> MDYKDDDDKLAAANSSIDLISTSLYKKAGFKGTNSVDMKVDRTKLKKTPTEAPADCRALIDKLKVCNDEQLLLELQQIKTWNIGKCELYHWVDLLDRFDGILADAGQTVENMSWMLVCDRPEREQLKMLLLAVLNFTALLIEYSFSRHLYSSIEHLTTLLASSDMQVVLAVLNLLYVFSKRSNYITRLGSDKRTPLLTRLQHLAESWGGKENGFGLAECCRDLHMMKYPPSATTLHFEFYADPGAEVKIEKRTTSNTLHYIHIEQLDKISESPSEIMESLTKMYSIPKDKQMLLFTHIRLAHGFSNHRKRLQAVQARLHAISILVYSNALQESANSILYNGLIEELVDVLQITDKQLMEIKAASLRTLTSIVHLERTPKLSSIIDCTGTASYHGFLPVLVRNCIQAMIDPSMDPYPHQFATALFSFLYHLASYDAGGEALVSCGMMEALLKVIKFLGDEQDQITFVTRAVRVVDLITNLDMAAFQSHSGLSIFIYRLEHEVDLCRKECPFVIKPKIQRPNTTQEGEEMETDMDGVQCIPQRAALLKSMLNFLKKAIQDPAFSDGIRHVMDGSLPTSLKHIISNAEYYGPSLFLLATEVVTVFVFQEPSLLSSLQDNGLTDVMLHALLIKDVPATREVLGSLPNVFSALCLNARGLQSFVQCQPFERLFKVLLSPDYLPAMRRRRSSDPLGDTASNLGSAVDELMRHQPTLKTDATTAIIKLLEEICNLGRDPK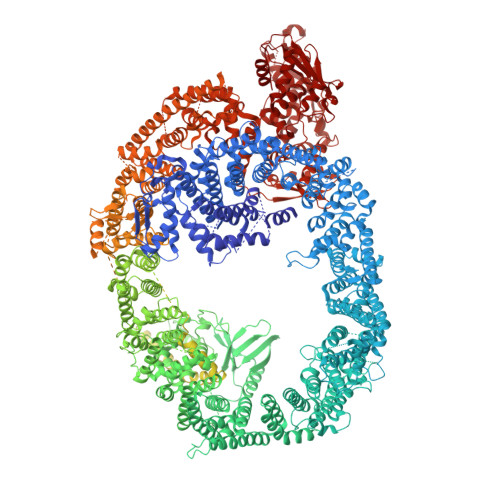YICQKPSIQKADGTATAPPPRSNHAAEEASSEDEEEEEVQAMQSFNSTQQNETEPNQQVVGTEERIPIPLMDYILNVMKFVESILSNNTTDDHCQEFVNQKGLLPLVTILGLPNLPIDFPTSAACQAVAGVCKSILTLSHEPKVLQEGLLQLDSILSSLEPLHRPIESPGGSVLLRELACAGNVADATLSAQATPLLHALTAAHAYIMMFVHTCRVGQSEIRSISVNQWGSQLGLSVLSKLSQLYCSLVWESTVLLSLCTPNSLPSGCEFGQADMQKLVPKDEKAGTTQGGKRSDGEQDGAAGSMDASTQGLLEGIGLDGDTLAPMETDEPTASDSKGKSKITPAMAARIKQIKPLLSASSRLGRALAELFGLLVKLCVGSPVRQRRSHHAASTTTAPTPAARSTASALTKLLTKGLSWQPPPYTPTPRFRLTFFICSVGFTSPMLFDERKYPYHLMLQKFLCSGGHNALFETFNWALSMGGKVPVSEGLEHSDLPDGTGEFLDAWLMLVEKMVNPTTVLESPHSLPAKLPGGVQNFPQFSALRFLVVTQKAAFTCIKNLWNRKPLKVYGGRMAESMLAILCHILRGEPVIRERLSKEKEGSRGEEDTGQEEGGSRREPQVNQQQLQQLMDMGFTREHAMEALLNTSTMEQATEYLLTHPPPIMGGVVRDLSMSEEDQMMRAIAMSLGQDIPMDQRAESPEEVACRKEEEERKAREKQEEEEAKCLEKFQDADPLEQDELHTFTDTMLPGCFHLLDELPDTVYRVCDLIMTAIKRNGADYRDMILKQVVNQVWEAADVLIKAALPLTTSDTKTVSEWISQMATLPQASNLATRILLLTLLFEELKLPCAWVVESSGILNVLIKLLEVVQPCLQAAKEQKEVQTPKWITPVLLLIDFYEKTAISSKRRAQMTKYLQSNSNNWRWFDDRSGRWCSYSASNNSTIDSAWKSGETSVRFTAGRRRYTVQFTTMVQVNEETGNRRPVMLTLLRVPRLNKNSKNSNGQELEKTLEESKEMDIKRKENKGNDTPLALESTNTEKETSLEETKIGEILIQGLTEDMVTVLIRACVSMLGVPVDPDTLHATLRLCLRLTRDHKYAMMFAELKSTRMILNLTQSSGFNGFTPLVTLLLRHIIEDPCTLRHTMEKVVRSAATSGAGSTTSGVVSGSLGSREINYILRVLGPAACRNPDIFTEVANCCIRIALPAPRGSGTASDDEFENLRIKGPNAVQLVKTTPLKPSPLPVIPDTIKEVIYDMLNALAAYHAPEEADKSDPKPGVMTQEVGQLLQDMGDDVYQQYRSLTRQSSDFDTQSGFSINSQVFAADGASTETSASGTSQGEASTPEESRDGKKDKEGDRASEEGKQKGKGSKPLMPTSTILRLLAELVRSYVGIATLIANYSYTVGQSELIKEDCSVLAFVLDHLLPHTQNAEDKDTPALARLFLASLAAAGSGTDAQVALVNEVKAALGRALAMAESTEKHARLQAVMCIISTIMESCPSTSSFYSSATAKTQHNGMNNIIRLFLKKGLVNDLARVPHSLDLSSPNMANTVNAALKPLETLSRIVNQPSSLFGSKSASSKNKSEQDAQGASQDSSSNQQDPGEPGEAEVQEEDHDVTQTEVADGDIMDGEAETDSVVIAGQPEVLSSQEMQVENELEDLIDELLERDGGSGNSTIIVSRSGEDESQEDVLMDEAPSNLSQASTLQANREDSMNILDPEDEEEHTQEEDSSGSNEDEDDSQDEEEEEEEDEEDDQEDDEGEEGDEDDDDDGSEMELDEDYPDMNASPLVRFERFDREDDLIIEFDNMFSSATDIPPSPGNIPTTHPLMVRHADHSSLTLGSGSSTTRLTQGIGRSQRTLRQLTANTGHTIHVHYPGNRQPNPPLILQRLLGPSAAADILQLSSSLPLQSRGRARLLVGNDDVHIIARSDDELLDDFFHDQSTATSQAGTLSSIPTALTRWTEECKVLDAESMHDCVSVVKVSIVNHLEFLRDEELEERREKRRKQLAEEETKITDKGKEDKENRDQSAQCTASKSNDSTEQNLSDGTPMPDSYPTTPSSTDAATSESKETLGTLQSSQQQPTLPTPPALGEVPQELQSPAGEGGSSTQLLMPVEPEELGPTRPSGEAETTQMELSPAPTITSLSPERAEDSDALTAVSSQLEGSPMDTSSLASCTLEEAVGDTSAAGSSEQPRAGSSTPGDAPPAVAEVQGRSDGSGESAQPPEDSSPPASSESSSTRDSAVAISGADSRGILEEPLPSTSSEEEDPLAGISLPEGVDPSFLAALPDDIRREVLQNQLGIRPPTRTAPSTNSSAPAVVGNPGVTEVSPEFLAALPPAIQEEVLAQQRAEQQRRELAQNASSDTPMDPVTFIQTLPSDLRRSVLEDMEDSVLAVMPPDIAAEAQALRREQEARQRQLMHERLFGHSSTSALSAILRSPAFTSRLSGNRGVQYTRLAVQRGGTFQMGGSSSHNRPSGSNVDTLLRLRGRLLLDHEALSCLLVLLFVDEPKLNTSRLHRVLRNLCYHAQTRHWVIRSLLSILQRSSESELCIETPKLTTSEEKGKKSSKSCGSSSHENRPLDLLHKMESKSSNQLSWLSVSMDAALGCRTNIFQIQRSGGRKHTEKHASGGSTVHIHPQAAPVVCRHVLDTLIQLAKVFPSHFTQQRTKETNCESDRERGNKACSPCSSQSSSSGICTDFWDLLVKLDNMNVSRKGKNSVKSVPVSAGGEGETSPYSLEASPLGQLMNMLSHPVIRRSSLLTEKLLRLLSLISIALPENKVSEAQANSGSGASSTTTATSTTSTTTTTAASTTPTPPTAPTPVTSAPALVAATAISTIVVAASTTVTTPTTATTTVSISPTTKGSKSPAKVSDGGSSSTDFKMVSSGLTENQLQLSVEVLTSHSCSEEGLEDAANVLLQLSRGDSGTRDTVLKLLLNGARHLGYTLCKQIGTLLAELREYNLEQQRRAQCETLSPDGLPEEQPQTTKLKGKMQSRFDMAENVVIVASQKRPLGGRELQLPSMSMLTSKTSTQKFFLRVLQVIIQLRDDTRRANKKAKQTGRLGSSGLGSASSIQAAVRQLEAEADAIIQMVREGQRARRQQQAATSESSQSEASVRREESPMDVDQPSPSAQDTQSIASDGTPQGEKEKEERPPELPLLSEQLSLDELWDMLGECLKELEESHDQHAVLVLQPAVEAFFLVHATERESKPPVRDTRESQLAHIKDEPPPLSPAPLTPATPSSLDPFFSREPSSMHISSSLPPDTQKFLRFAETHRTVLNQILRQSTTHLADGPFAVLVDYIRVLDFDVKRKYFRQELERLDEGLRKEDMAVHVRRDHVFEDSYRELHRKSPEEMKNRLYIVFEGEEGQDAGGLLREWYMIISREMFNPMYALFRTSPGDRVTYTINPSSHCNPNHLSYFKFVGRIVAKAVYDNRLLECYFTRSFYKHILGKSVRYTDMESEDYHFYQGLVYLLENDVSTLGYDLTFSTEVQEFGVCEVRDLKPNGANILVTEENKKEYVHLVCQMRMTGAIRKQLAAFLEGFYEIIPKRLISIFTEQELELLISGLPTIDIDDLKSNTEYHKYQSNSIQIQWFWRALRSFDQADRAKFLQFVTGTSKVPLQGFAALEGMNGIQKFQIHRDDRSTDRLPSAHTCFNQLDLPAYESFEKLRHMLLLAIQECSEGFGLA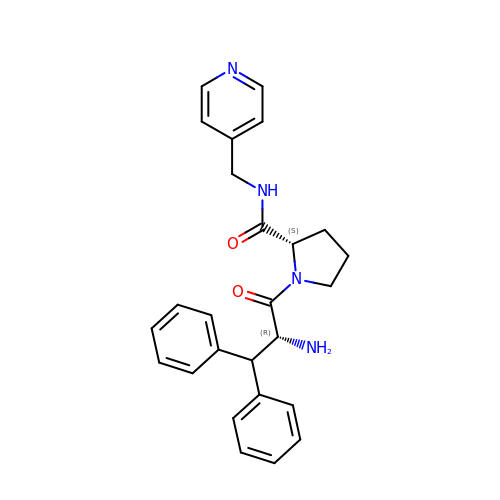(2~{S})-1-[(2~{R})-2-azanyl-3,3-diphenyl-propanoyl]-~{N}-(pyridin-4-ylmethyl)pyrrolidine-2-carboxamide | C26 H28 N4 O2 | DPXLHPWLQSWEQB-LADGPHEKSA-N> NEDMPVERILEAELAVEPKTETYVEANMGLNPSSPNDPVTNICQAADKQLFTLVEWAKRIPHFSELPLDDQVILLRAGWNELLIASFSHRSIAVKDGILLATGLHVHRNSAHSAGVGAIFDRVLTELVSKMRDMQMDKTELGCLRAIVLFNPDSKGLSNPAEVEALREKVYASLEA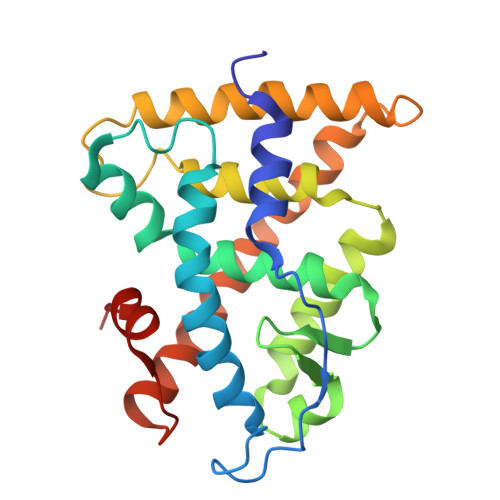YCKHKYPEQPGRFAKLLLRLPALRSIGLKCLEHLFFFKLIGDTPIDTFLMEMLEAPHQMT> SLYKGYLIDLDGTIYKGKDRIPAGETFVHELQKRDIPYLF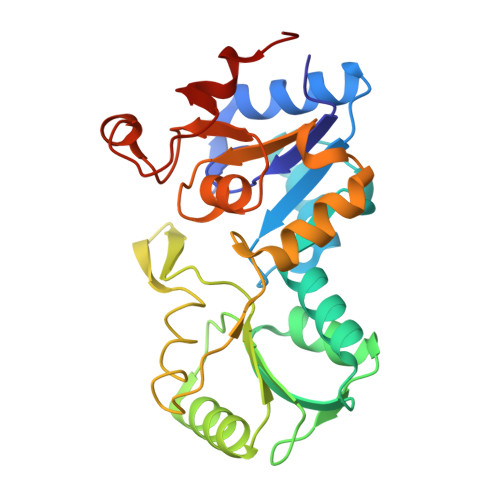VTNNTTRTPESVKEMLAQNFNIDTPLSTVYTATLATIDYMNDLGLEKTVYVVGEAGLKEAIKAAGYVEDKEKPAYVVVGLDWQVDYEKFATATLAIQKGAHFIGTNPDLNIPTERGLLPGAGSLITLLEVATRVKPVYIGKPNAIIMDKAVEHLGLEREELIMVGDNYLTDIRAGIDNGIPTLLVTTGFTKAEEVAGLPIAPTHVVSSLAEWDFDEN> GPVKTQEDLLPLVPEQVFVEMYEDMARRQTIEALVPAWDSDIIFKCLCYFHTLYPGLIPLETFPPATIFNFKQKII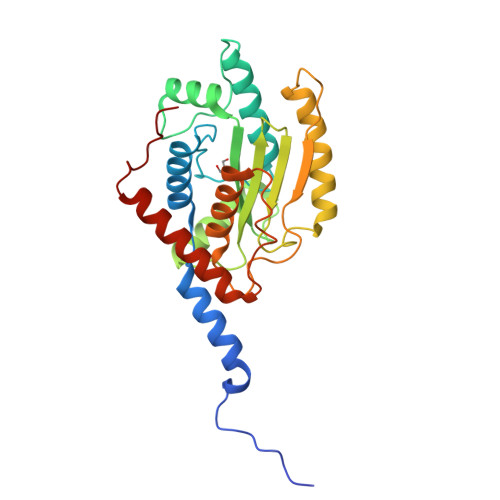SILEDKKAVLRGEPIKGPLPICCSKENYRRHLQRTTLLPVFMWYHPTPKTLSDTMQTMKQLAIKGSVGASHWLLVIVDIQARRLVYFDSLYNYVMPPENMKKELQSFAQQLDQVYPAYDSKKFSVKIAAKEVIQRGSGSSCGAWCCQFLHWYLKDPLTDALNDLPVDSVERHENLASFVQACEAAVQDLPELSWPEA> MATAGNPWGWFLGYLILGVAGSLVSGSCSQIINGEDCSPHSQPWQAALVMENELFCSGVLVHPQWVLSAAHCFQNSYTIGLGLHSLEADQEPGSQMVEASLSVRHPEYNRPLLANDLMLIKLDESVSESDTIRSISIASQCPTAGNSCLVSGWGLLANGRMPTVLQCVNVSVVSEEVCSKLYDPLYHPSMFCAGGGHDQKDSCNGDSGGPLICNGYLQGLVSFGKAPCGQVGVPGVYTNLCKFTEWIEKTVQAS;> PQFGLFSKYRTPNCRRYSIHGCNRMYAPVCGSDMSTYANECTLCMKIREGGHNIKIIKNGPCGAS

By screening of scaffolds which met requirements as therapeutic proteins, we selected serine protease inhibitor Kazal-type 2 (SPINK2) as a protein scaffold, followed by constructing an engineered SPINK2 library. SPINK2 comprises a constrained region containing disulfide bonds, and a flexible loop region. Using a series of phage display screening experiments and a diverse engineered SPINK2 library, we succeeded in acquiring quite specific inhibitors for every target protease tested with sub-nanomolar Ki values and picomolar KD values. Further, generation of a crystal structure provided insights into the mechanism underlying the high affinity specific binding of those inhibitors for their target molecules, suggesting that the engineered SPINK2 inhibitors preferentially bind to the groove of target proteases via the engineered flexible loop, supported by its constrained structure.

In addition, the KLK4/8 dual inhibitor, K41043 had IC50 values of 2.1 and 14 nM for KLK4 and KLK8, respectively. The randomized region of K41043 directed to the catalytic pocket of KLK4, and K41043 residue Asn23 formed a hydrogen bond with the catalytic His71 of KLK4. The S1 pocket of KLK4 was deeply buried by K41043 residue Arg24, forming a salt bridge and hydrogen bonds. In addition, K41043 formed a 310-helix at the randomized region of the crystal structure, whereas this was not observed in the wild-type SPINK2. In contrast, there were conformational differences between wild-type SPINK2 and K41043, which were primarily observed the in randomized region; the maximum distance between them was 11.4 Å (Cαs). There were few conformational differences in KLK4 with or without K41043; the root-mean-square deviation value between them was 0.346 Å from 190 Cαs. The binding loop of K41043 was entirely buried in this large area, providing a high level of conformational complementarity, and there were no water molecules within 7 Å of the catalytic His71 of KLK4. In the KLK4–K41043 co-crystal structure, there were no water molecules within 7 Å from the catalytic His71 of KLK4. This may be because binding of K41043 to KLK4 excluded the water molecules essential for protease turnover, hence K41043 acted as an inhibitor, but not as a substrate. It revealed that 25 residues of KLK4 within 4 Å from K41043 were located not only in the S1 pocket, including the catalytic residues (His71 and Ser207), but also in a surface distant from the S1 pocket. In the KLK4–K41043 structure, the entire interaction surface area was 863.3 Å2, and included salt bridges, hydrogen bonds, and hydrophobic contacts.The human nucleoporin Nup98 forms fusion proteins in certain types of malignant leukaemia, is a critical component of the permeability barrier of the nuclear pore complex and is mislocalized in cytosolic deposits in Alzheimer’s disease. Key to these Nup98 activities is its large FG-repeat domain with a high number of FG motifs. The most aggregation-prone segment comprises residues 85–124 (named Nup98FG85). All four fibril types display a parallel in-register β-structure comprising short and kinked β-strands.

To gain insight into the molecular organization of cohesive FG-repeat interactions, Nup98FG85 was allowed to aggregate in pure water. EM revealed the formation of well-defined and mostly separated amyloid fibrils. Using cryo-EM, we determined the structures of four different fibril polymorphs (pm1–pm4). Polymorphs pm2 and pm3, which are almost equally populated, were solved at a resolution of 3.3 and 2.8 Å, respectively, and are formed by two protofilaments. The most common motif shared by the four polymorphs is a 13-residue β-turn/β-arch structure. A leucine-phenylalanine pair (L91-F92) is located at the tip of the β-turn, with both side chains pointing away from the turn. The other LF motifs in the four fibril structures show a very similar structure. In all four Nup98FG85 fibril structures, side chains stacked along the fibril axes build glutamine and asparagine ladders (top). Most of the stabilizing interactions arise where there are clusters of two to four phenylalanine rings and one or more leucine side chains. We obtained values of approximately −20 kcal mol–1 per chain for the four Nup98FG85 fibril structures.

>[22x]TGTANTLFGTASTGTSLFSSQNNAFAQNKPTGFGNFGTST>[2x]M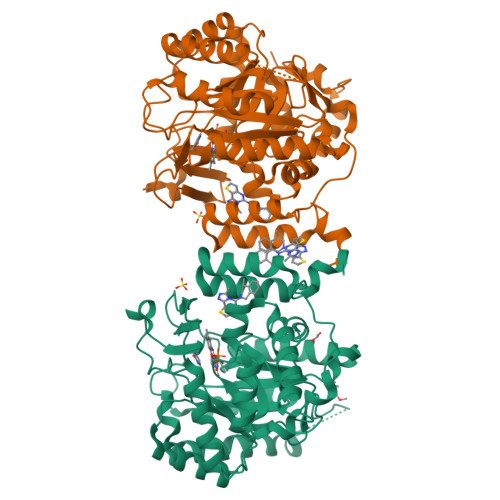GHHHHHHAENLYFQGADPFESYNPEFFLYDIFLKFCLKYIDGEICHDLFLLLGKYNILPYDTSNDSIYACTNIKHLDFINPFGVAAGFDKNGVCIDSILKLGFSFIEIGTITPRGQTGNAKPRIFRDVESRSIINSCGFNNMGCDKVTENLILFRKRQEEDKLLSKHIVGVSIGKNKDTVNIVDDLKYCINKIGRYADYIAINVSSPNTPGLRDNQEAGKLKNIILSVKEEIDNLEKNNIMNDEFLWFNTTKKKPLVFVKLAPDLNQEQKKEIADVLLETNIDGMIISNTTTQINDIKSFENKKGGVSGAKLKDISTKFICEMYNYTNKQIPIIASGGIFSGLDALEKIEAGASVCQLYSCLVFNGMKSAVQIKRELNHLLYQRGYYNLKEAIGRKHSKS The Mad1‐Mad2 complex, which is required to catalyse MCC formation, is targeted to kinetochores through a direct interaction with the phosphorylated conserved domain 1 (CD1) of Bub1. Mad1CTD is comprised of an N‐terminal elongated coiled‐coil, followed by a globular head domain featuring a conserved RWD (RING, WD40, DEAD) domain. Each monomer contains a long N‐terminal α‐helix (α1) forming the stem, followed by an antiparallel β‐sheet of four β‐strands (β1–4), a short helix (α2) and two C‐terminal helices (α3/α4). Bub1CD1 is largely a single α‐helix, consisting of almost four turns.

In each case, the asymmetry of the homodimer was retained. Crystallization of Mad1CTD‐Bub1CD1 with a twofold higher peptide concentration of 5 mM led to a lower resolution structure most likely due to the twofold increase in DMSO. However, the differential occupancy, although reduced, was still observed in this structure (Fig EV2B). Thus, this peptide is likely to bind with higher affinity and to represent the single binding peptide in solution as detected by NMR, ITC and AUC analyses. This model is supported by our Mad1CTD‐Bub1CD1 structures from various space groups where higher occupancy of the second Bub1CD1 peptide correlates with a more symmetric Mad1CTD dimer (Fig EV4). Alignment of all four Mad1CTD homodimers from the three different space group structures displays the extent of the flexibility within the Mad1CTD coiled‐coil and head domain (Fig EV4G).

>[2x]SSKEVAELKKQVESAELKNQRLKEVFQTKIQEFRKACYTLTGYQIDITTENQYRLTSLYAEHPGDCLIFKATSPSGSKMQLLETEFSHTVGELIEVHLRRQDSIPAFLSSLTLELFSRQTVA;>[2x]KVQPSPTVHTKEALGFIMNMFQAPTS> AARATVAGGGRLMDRIRKWYYNAAGFNKYGLMRDDTLYEDDDVKEALKRLPEDLYNERMFRIKRALDLSLKHRILPKEQWVK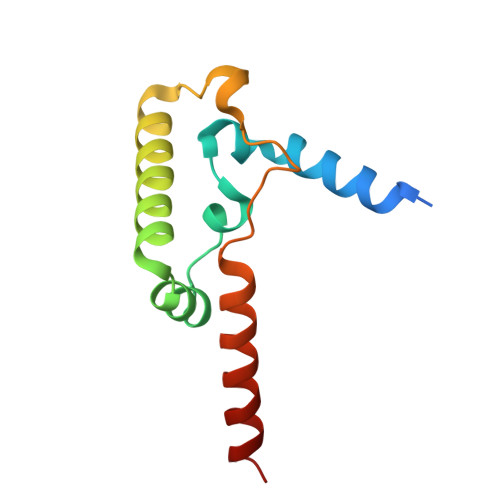YEEDKPYLEPYLKEVIRERLEREAWNKK> MKYDTSELCDIYQEDVNVVEPLFSNFGGRASFGGQIITVKCFEDNGLLYDLLEQNGRGRVLVVDGGGSVRRALVDAELARLAVQNEWEGLVIYGAVRQVDDLEELDIG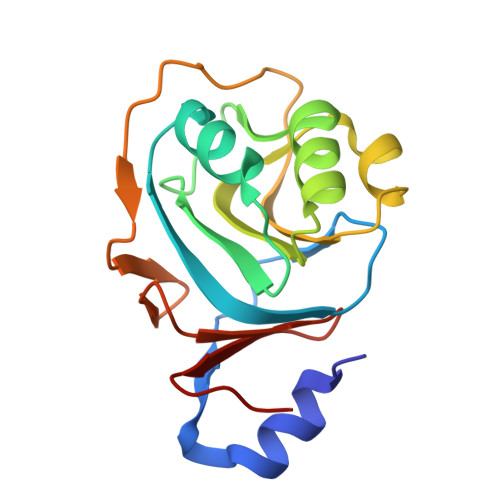IQAMAAIPVGAAGEGIGESDVRVNFGGVTFFSGDHLYADNTGIILSEDPLDIE> GMSDPRTQP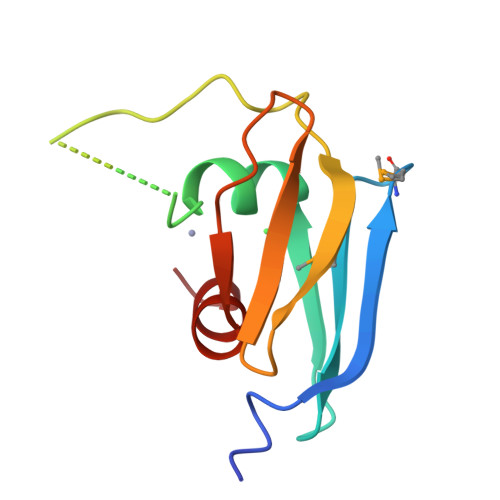LEIRPLMISRVMEVDWADGHTSRLTFEHLRVECPCAECKGHTPDQAQIVTGKEHVSVVEVVPVGHYAVQLHFSDGHNTGIFTWEYLRRLDAE> GMAQRSILVGQIWHEGHSFNPILTREKDFLFLRGEAVLEEARASSTALSGIVKTAEALGYRCVPSISARARPGGAIEQKVFDNIVDEFVQAARMQDFDAICLDLHGATLAEHTLDTEGYLLSRLREVVGNDIMISLALDLHAYLTPQMVEQATIITSFRTTPHADIEETGVRAMTLLDSLSNETRPPRAIYSLIPFLT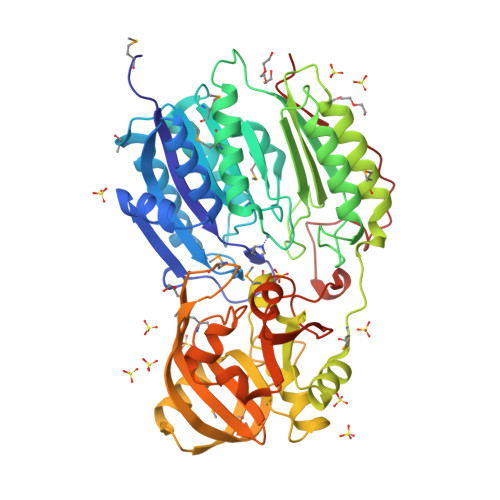RGNDETWSGPLAEIGAAADRWRARSDVVDLSIFNVHPFLDVPGYGQVVLAYDNGSGAAIDACRDLSDMLWKARDEFQEQLMSVDKALEIARTSRQLLALGDQGDRVMGAGPGDSPEIARVALEHFPGLKVAVPVYDPQAVRTAREAGENATVRMAVGGAFTHSVAPLERDWTVRKLCRARFTNIGPYMAGTEADFGDAAVLTCDAVTVIVTTMAPNVHDPAFYEAVGVPLASQQAVVARAANHYKLSFADIARTITVDTPGLTAFKPHQFPFTQARPFYPLDIVQWSFAPLECNKVG3-{2-[(E)-iminomethyl]-6-propylpyrimidin-4-yl}-N,N-dimethyl-5-(trifluoromethyl)benzamide | C18 H19 F3 N4 O | 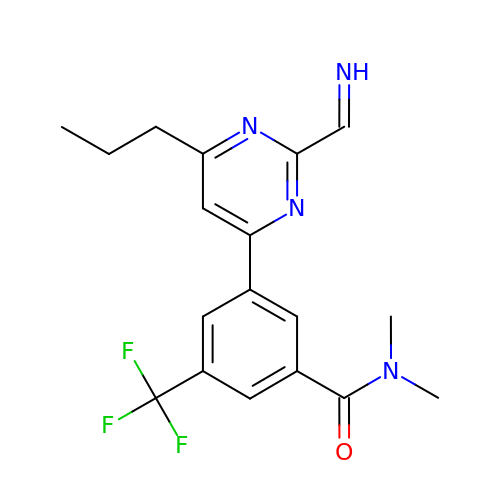FLPAOFVJMBOQGB-LSHDLFTRSA-N>MQPSFRIVADGTDVTQRLNDRLLKLTLLDKPGMESDSLTLRIDDRDGQVALPRRGAVLEVHLGYAGEPLMRMGRFTVDTLQWAGPPDCLTVTAKAGDMRGSGKTIR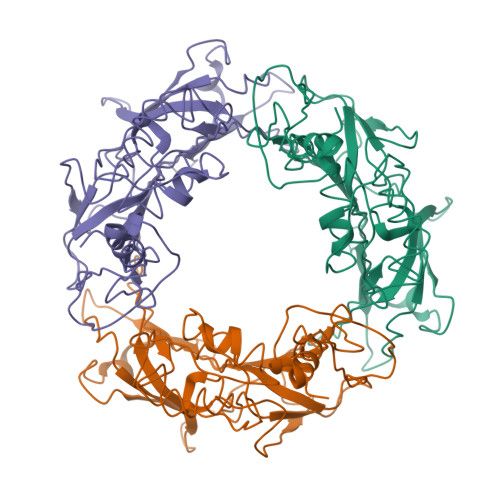SGGWEGTTLAQVCRDVGARNGWRVECPLQVAIARVDQVNESDYHFVTRLARQYDCTAKLAEGMLMVLPRQSGQSATGRRIEPLVLGRADVGSFDVTFDDRSLMRTVKTRYQLPGSGEVKSVELKNPKAPATAMGEHVDRHLYTSRGEAEQAAKARLASFSRSSASVRLELPGRGDLFAERSLLLQGFKAGIDGEFLIDSVEHTYSSSGWTTVVQCNGGRGGKG[3x]> ACTKNAIAQTGFNKDKYFNGDVWYVTDYLDLEPDDVPKRYCAALAAGTASGKLKEALYHYDPKTQDTFYDVSELQVESLGKYTANFKKVDKNGNVKVAVT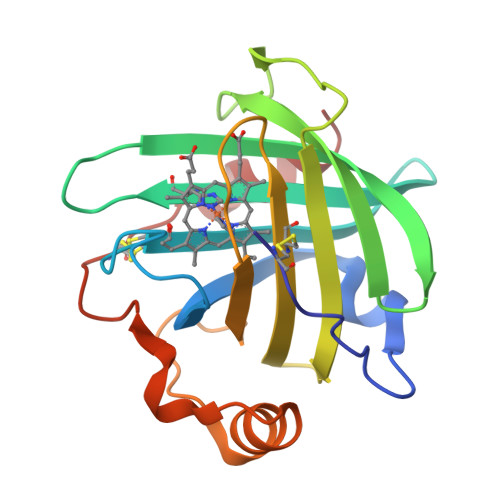AGNYYTFTVMYADDSSALIHTCVHKGNKDLGDVYAVLNRNKDAAAGDKVKSAVSAATLEFSKFISTKENNCAYDNDSLKSLLTK> SSVPLEWPLSSQSGSYELRIEVQPKPHHRAHYETEGSRGAVKAPTGGHPVVQLHGYMENKPLGLQIFIGTADERILKPHAFYQVHRITGKTVTTTSYEKIVGNTKVLEIPLEPKNNMRATIDCAGILKLRNADIELRKGETDIGRKNTRVRLVFRVH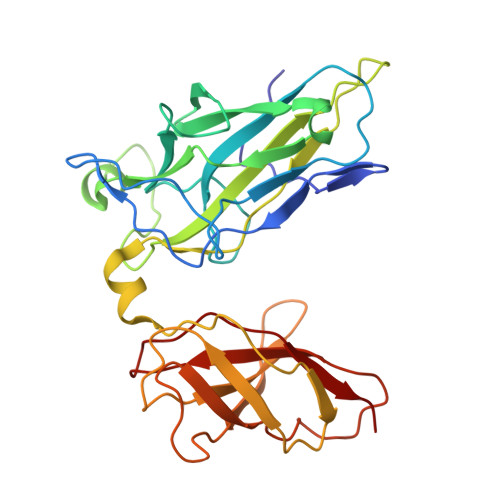IPESSGRIVSLQTASNPIECSQRSAHELPMVERQDTDSCLVYGGQQMILTGQNFTSESKVVFTEKTTDGQQIWEMEATVAAAAAAPNMLFVEIPEYRNKHIRTPVKVNFYVINGKRKRSQPQHFTYHPV>[2x]GAMGGEEVSEEGFQIPATITERYKVGRTIGDGNFAVVKECVERSTAREYALKIIKKSKCRGKEHMIQNEVSILRRVKHPNIVLLIEEMDVPTELYLVMELVKGGDLFDAITSTNKYTERDASGMLYNLASAIKYLHSLNIVHRDIKPENLLVYEHQDGSKSLKLGDFGLATIVDGPLYTVCGTPTYVAPEIIAETGYGLKVDIWAAGVITYILLCGFPPFRGSGDDQ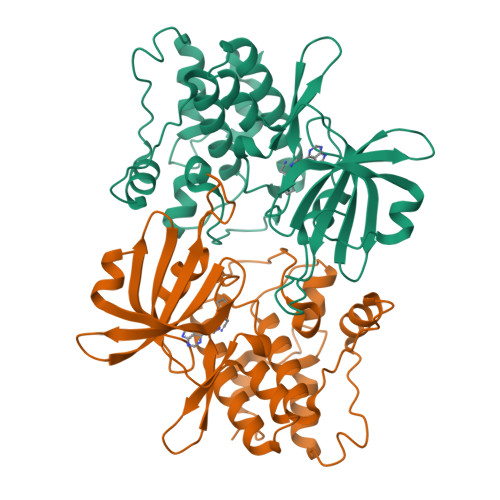EVLFDQILMGQVDFPSPYWDNVSDSAKELITMMLLVDVDQRFSAVQVLEHPWVND>MADLPISLLQTLAYKQPLGRNSRIVHFTDGALFPVVAFGDNHSTSELYIAVRGDHRDLMSPDVRDSYALTGDDHKVWGATHHTYYVEGAPKKPLKFNVKTRTDLTILPVADVFWRADGSADVDVVWNDMPAVAGQSSSIALALASSLPFVPKAAYTGCLSGTNVQPVQFGNLKARAAHKIGLPLVGMTQDGGEDTRICTLDDAADHAFDSMES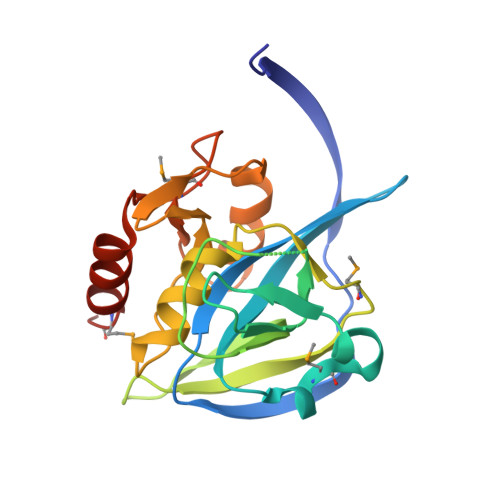TVTR[2x]> TLVEQILAEFQLQEEDLKKVMRRMQKEMDRGLRLE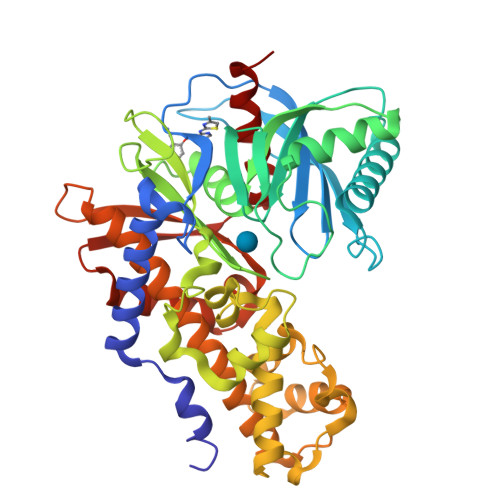THEEASVKMLPTYVRSTPEGSEVGDFLSLDLGGTNFRVMLVKVGEGEEGQWSVKTKHQMYSIPEDAMTGTAEMLFDYISECISDFLDKHQMKHKKLPLGFTFSFPVRHEDIDKGILLNWTKGFKASGAEGNNVVGLLRDAIKRRGDFEMDVVAMVNDTVATMISCYYEDHQCEVGMIVGTGCNACYMEEMQNVELVEGDEGRMCVNTEWGAFGDSGELDEFLLEYDRLVDESSANPGQQLYEKLIGGKYMGELVRLVLLRLVDENLLFHGEASEQLRTRGAFETRFVSQVESDTGDRKQIYNILSTLGLRPSTTDCDIVRRACESVSTRAAHMCSAGLAGVINRMRESRSEDVMRITVGVDGSVYKLHPSFKERFHASVRRLTPSCEITFIESEEGSGRGAALVSAVACKKAC>[2x]EEDKAYWNKDAQDALDKQLGIKLREKQAKNVIFFLGDGMSLSTVTAARIYKGGLTGKFEREKISWEEFDFAALSKTYNTDKQVTDSAASATAYLTGVKTNQGVIGLDANTVRTNCSYQLDESLFTYSIAHWFQEAGRSTGVVTSTRVTHATPAGTYAHVADRDWENDSDVVHDREDPEICDDIAEQLVFREPGKNFKVIMGGGR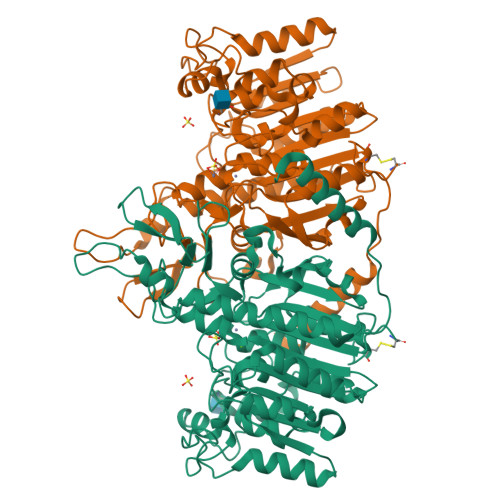RGFFPEEALDIEDGIPGEREDGKHLITDWLDDKASQGATASYVWNRDDLLAVDIRNTDYLMGLFSYTHLDTVLTRDAEMDPTLPEMTKVAIEMLTKDENGFFLLVEGGRIDHMHHANQIRQSLAETLDMEEAVSMALSMTDPEETIILVTADHGHTLTITGYADRNTDILDFAGISDLDDRRYTILDYGSGPGYHITEDGKRYEPTEEDLKDINFRYASAAPKHSVTHDGTDVGIWVNGPFAHLFTGVYEENYIPHALAYAACVGTGRTFCDEK>[4x]GSHMSASAEPESDVKGRILDAAADAFMLRGFANTTIDDIADDVGATKGLIYYHFRSKFDIFLAVYEDGMRRVRERVEPYVGAPGTGRQRLVAMSVAHVENLMIDLGYHHVVHQGVRDQASTALKVRQRDALAALNELRRDYERMFHHVITEGIADGSLRNVDDALATRTLLSNLNAVDVWYRKIEGQTEKEVHDLASQVVDLLIGGIGATAD

The mycobacterial repressor, DarR, a TetR family regulator (TFR), was the first transcription regulator shown to bind c-di-AMP. Recently, DarR, a 201 residue, TFR regulator of a putative MDR transporter, Ms5347, in Mycobacteria was discovered and represents the focus of this work. Structures of TFR proteins reveal that they share a two-domain architecture with an N-terminal DNA-binding domain and a C-terminal inducer binding/dimerization domain. The DarR N-terminal domain consists of helices 1-3 and the dimer domain is comprised of helices α4-α9. In DarR, dimerization is mediated by helices α8 and α9, which interact with α8´ and α9´ (where the prime indicates the other subunit in the dimer) to form a four-helix bundle dimerization module.

To elucidate the structural mechanism of c-di-AMP binding we obtained the Rhodococcus sp. USK13 DarR-c-di-AMP structure to 2.45 Å resolution. The structure revealed no density for c-di-AMP in the inducer binding pocket, but density for a di-adenine nucleotide was observed near the four-helix bundle module of DarR, with the nucleotide making contacts to both subunits of the dimer. The density for the adenine moieties was well resolved while the density for the phosphate groups was less clear. Hence, a di-adenine nucleotide was fitted to the map. In the structure, the dinucleotide is wedged within the long loop between helices α8 and α9 of one DarR subunit and also contacts residues from the N-terminus of α8´ from the other subunit. In this interaction, only one of the adenine bases is bound within each pocket and the other adenine base is solvent exposed. Each of the exposed adenine bases inserts into the binding pocket of an adjacent DarR dimer, leading to DarR polymer contacts in the crystal. In addition to Gln184 and Arg179 both adenine moieties are contacted by the side chains of Trp177, Tyr178, Ile181 and Leu192 from one DarR subunit and Asp159 Leu162 and Arg165 from the other subunit. As noted, the density for the phosphates are weak and indeed, there are no phosphate contacts from DarR.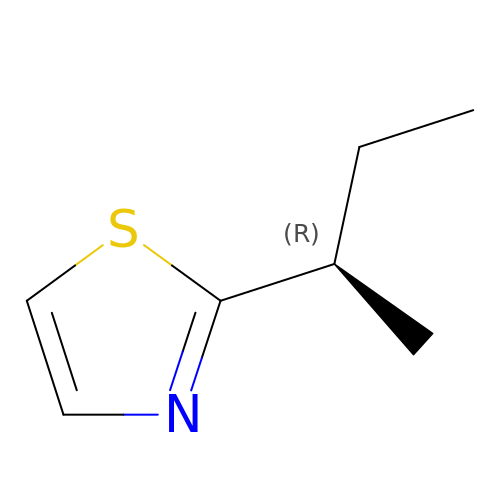2-(SEC-BUTYL)THIAZOLE | C7 H11 N S | MHJSWOZJMPIGJQ-ZCFIWIBFSA-N Streptozotocin | C8 H15 N3 O7 | 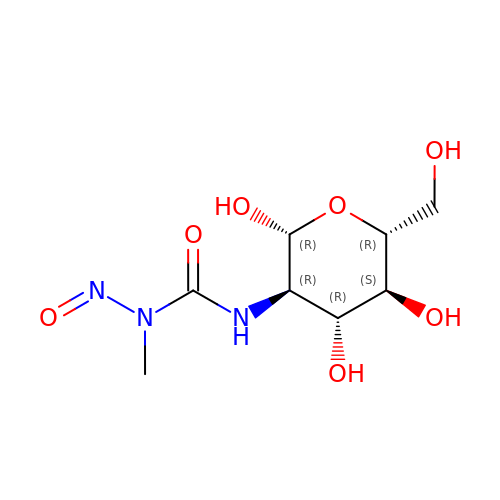ZSJLQEPLLKMAKR-NYMZXIIRSA-N>CPRFLKVKNWETEVVLTDTLHLKSTLETGCTEYICMGSIMHPSQHARRPEDVATKDQLFPLAKEFIDQYYSSIKRFGSKAHMERLEEVNKEIDTTSTYQLKDTELIYGAKHAWRNASRCVGRIQWSKLQVFDARDCTTAHGMFNYICNHVKYATNKGNLRSAITIFPQRTDGKHDFRVWNSQLIRYAGYKQPDGSTLGDPANVQFTEICIQQGWKPPRGRFDVLPLLLQANGNDPELFQIPPELVLEVPIRHPKFEWFKDLGLKWYGLPAVSNMLLEIGGLEFSACPFSGWYMGTEIGVRDYCDNSRYNILEEVAKKMNLDMRKTSSLWKDQALVEINIAVLYSFQSDKVTIVDHHSATESFIKHMENEYRCRGGCPADWVWIVPPMSGSITPVFHQEMLNYRLTPSFEYQPDPWNTHVWKLV[2x]

Nitric oxide (NO) is an important signaling molecule critical in the cardiovascular, neuronal, and immune systems. The enzyme responsible for generating NO is nitric oxide synthase (NOS), a P450-like heme thiolate enzyme that oxidizes l-arginine to NO and L-citrulline. Humans and other mammals express three different NOS isoforms: endothelial NOS (eNOS), neuronal NOS (nNOS), and inducible NOS (iNOS). nNOS is an important therapeutic target since the overproduction of NO by nNOS in the brain is associated with a number of neurodegenerative diseases. Thus, nNOS is an attractive target for therapeutic intervention. In our efforts to develop inhibitors selective for neuronal nitric oxide synthase (nNOS) over endothelial nitric oxide synthase (eNOS), we found that nNOS can undergo conformational changes in response to inhibitor binding that does not readily occur in eNOS. Here, we used a combination of crystallography, mutagenesis, and computational methods to better understand the structural basis for these differences in NOS inhibitor binding.

We first observed protein backbone structural changes with compound 3, followed by observations of the same structural changes in nNOS with many other inhibitors (12 cases in hnNOS and four cases in rnNOS, unpublished results). Compound 4 is a typical example, as shown in Figure 8, where the inhibitor can bind both to the active site and to the BH4 site in hnNOS, triggering backbone changes, but only one inhibitor binds to the active site in heNOS and does not induce backbone changes. Indeed, in the various structures with two inhibitor molecules bound, the inhibitor bound in the active site contacts the inhibitor in the BH4 pocket. Inhibitor binding in the BH4 site often requires a significant conformational rearrangement near the dimer interface to provide room for the second inhibitor molecules. We therefore hypothesized that the weaker dimer interface interactions in hnNOS allow the 598–611 region a wider range of dynamic flexibility than the corresponding region in heNOS. In addition, mutating the active site Glu to Gln in nNOS resulted in the same conformational change that results from two inhibitors binding. This suggests that when two inhibitors bind, the first one enters the active site and hydrogen bonds with the active site Glu, lowering the energetic barrier to the conformational change required to bind the second molecule that displaces BH4.>[4x]MLSRKGIIPEEYVLTRLAEDPTEPRYRTRERRARFVSKKGNCNVAHKNIREQGRFLQDVFTTLVDLKWPHTLLIFTMSFLCSWLLFAMVWWLIAFAHGDLAPGEGTNVPCVTSIHSFSSAFLFSIEVQVTIGFGGRMVTEECPLAILILIVQNIVGLMINAIMLGCIFMKTAQAHRRAETLIFSKHAVITPRHGRLCFMLRVGDLRKSMIISATIHMQVVRKTTSPEGEVVPLHQVDIPMENGVGGNSIFLVAPLIIYHVIDSNSPLYDLAPSDLHHHQDLEIIVILEGVVETTGITTQARTSYLADEILWGQRFVPIVAEEDGRYSVDYSKFGNTVKVPTPLCTARQLDEDRSLLDALTLASSRGPLRKRSVAVAKAKPKFSISPDSLS;>DYKDDDDKMPLAFCGTENHSAAYRVDQGVLNNGCFVDALNVVPHVFLLFITFPILFIGWGSQSSKVHIHHSTWLHFPGHNLRWILTFILLFVLVCEIAEGILSDGVTESRHLHLYMPAGMAFMAAITSVVYYHNIETSNFPKLLIALLIYWTLAFITKTIKFVKFYDHAIGFSQLRFCLTGLLVILYGMLLLVEVNVIRVRRYIFFKTPREVKPPEDLQDLGVRFLQPFVNLLSKGTYWWMNAFIKTAHKKPIDLRAIAKLPIAMRALTNYQRLCVAFDAQARKDTQSPQGARAIWRALCHAFGRRLILSSTFRILADLLGFAGPLCIFGIVDHLGKENHVFQPKTQFLGVYFVSSQEFLGNAYVLAVLLFLALLLQRTFLQASYYVAIETGINLRGAIQTKIYNKIMHMSTSNLSMGEMTAGQICNLVAIDTNQLMWFFFLCPNLWTMPVQIIVGVILLYYILGVSALIGAAVIILLAPVQYFVATKLSQAQRTTLEHSNERLKQTNEMLRGMKLLKLYAWESIFCSRVEVTRRKEMTSLRAFAVYTSISIFMNTAIPIAAVLITFVGHVSFFKESDLSPSVAFASLSLFHILVTPLFLLSSVVRSTVKALVSVQKLSEFLSSAEIREEQCAPREPAPQGQAGKYQAVPLKVVNRKRPAREEVRDLLGPLQRLAPSMDGDADNFCVQIIGGFFTWTPDGIPTLSNITIRIPRGQLTMIVGQVGCGKSSLLLATLGEMQKVSGAVFWNSNLPDSEGEDPSSPERETAAGSDIRSRGPVAYASQKPWLLNATVEENITFESPFNKQRYKMVIEACSLQPDIDILPHGDQTQIGERGINLSGGQRQRISVARALYQQTNVVFLDDPFSALDVHLSDHLMQAGILELLRDDKRTVVLVTHKLQYLPHADWIIAMKDGTIQREGTLKDFQRSECQLFEHWKTLMNRQDQELEKETVMERKASEPSQGLPRAMSSRDGLLLDEEEEEEEAAESEEDDNLSSVLHQRAKIPWRACTKYLSSAGILLLSLLVFSQLLKHMVLVAIDYWLAKWTDSALVLSPAARNCSLSQECDLDQSVYAMVFTLLCSLGIVLCLVTSVTVEWTGLKVAKRLHRSLLNRIILAPMRFFETTPLGSILNRFSSDCNTIDQHIPSTLECLSRSTLLCVSALTVISYVTPVFLVALLPLAVVCYFIQKYFRVASRDLQQLDDTTQLPLVSHFAETVEGLTTIRAFRYEARFQQKLLEYTDSNNIASLFLTAANRWLEVCMEYIGACVVLIAAATSISNSLHRELSAGLVGLGLTYALMVSNYLNWMVRNLADMEIQLGAVKRIHALLKTEAESYEGLLAPSLIPKNWPDQGKIQIQNLSVRYDSSLKPVLKHVNTLISPGQKIGICGRTGSGKSSFSLAFFRMVDMFEGRIIIDGIDIAKLPLHTLRSRLSIILQDPVLFSGTIRFNLDPEKKCSDSTLWEALEIAQLKLVVKALPGGLDAIITEGGENFSQGQRQLFCLARAFVRKTSIFIMDEATASIDMATENILQKVVMTAFADRTVVTIAHRVHTILSADLVMVLKRGAILEFDKPETLLSQKDSVFASFVRADK[4x]

Subsequent cloning and characterization revealed the β-cell KATP channel as a complex of two proteins: a potassium channel Kir6.2 of the inwardly rectifying K+ channel family, and a sulfonylurea receptor SUR1, a member of the ATP binding cassette (ABC) transporter protein family. Physiological activity of KATP channels is determined primarily by the relative concentrations of ATP and ADP: ATP inhibits, whereas MgADP stimulates channel activity. As KATP channels set the β-cell membrane potential, this regulation by nucleotides endows them the ability to sense metabolic changes and translate those into changes in membrane excitability, which ultimately initiates or stops insulin secretion. Importantly, KATP channels are the targets of sulfonylureas, one of the most commonly prescribed treatments for type 2 diabetes, which stimulate insulin secretion by inhibiting channel activity.

The structure shows that the KATP channel is an octamer built around a Kir6.2 tetramer with each subunit complexed to one SUR1. The complex is ~200 Å in width in the longest dimension and ~125 Å in height, and is shaped like a propeller with the Kir6.2 pore and TMD0 forming a compact central core and the SUR1-ABC core structure forming the blades. In our structure, TMD0-L0 sits in between the SUR1 and Kir6.2 subunits and is the primary point of contact between the SUR1-ABC core and Kir6.2. A comparison of closed (Kir3.2 apostate) and open (Kir3.2-R201A + PIP2) G-loop structures in relation to Kir6.2 suggests that this gate is also closed. Together, these observations indicate a closed channel structure, which is expected since the sample contained saturating concentrations of inhibitory ATP and GBC. An overview of the ATP binding site from the side, and from the top, with ATP colored in red, illustrates that the pocket is at the interface of adjacent Kir6.2 N and C domains. A close-up view shows that the docked ATP is surrounded by residues I182, L205, Y330, F333, and G334 from the same subunit, and R50 from the adjacent subunit. In our structure, we see that the density corresponding to ATP is located on the periphery of the Kir6.2 cytoplasmic domain, and traversed by the N-terminal segment of L0 of SUR1 immediately following TMD0, with the Cα of K205 coming within only ~10 Å of the site. Overall, the SUR1-ABC core is in an inward-facing conformation, with the NBDs clearly separated. However, in contrast to other ABC exporters of known structure whereby transporter halves are related by either a true or a pseudo two-fold symmetry axis, depending on whether the two halves are identical or not, we find a clear rotation and a translation of TMD1-NBD1 relative to TMD2-NDB2, such that TMD1-NBD1 is ~15° off the symmetry axis and is translated by ~10 Å horizontally (relative to the membrane).>[2x]LLHKRVVLASASPRRQEIL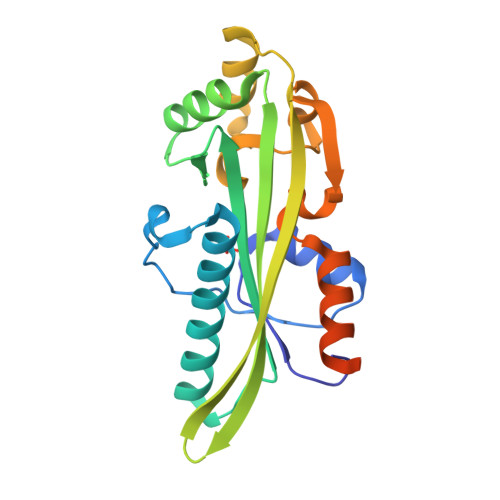SNAGLRFEVVPSKFKEKLDKASFATPYGYAMETAKQKALEVANRLYQKDLRAPDVVIGADTIVTVGGLILEKPVDKQDAYRMLSRLSGREHSVFTGVAIVHCSSKDHQLDTRVSEFYEETKVKFSELSEELLWEYVHSGEPMDKAGGYGIQALGGMLVESVHGDFLNVVGFPLNHFCKQLVKLYYPPRPEDLRRSVKHDSIPAADTFEDLS> AEQVTKSVLFVCLGNICRSPIAEAVFRKLVTDQNISDNWVIDSGAVSDWNVGRSPDPRAVSCLRNHGINTAHKARQVTKEDFVTFDYILCMDESNLRDLNRKSN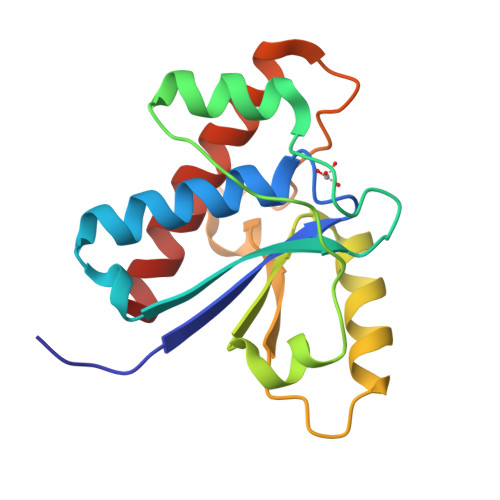QVKNCRAKIELLGSYDPQKQLIIEDPYYGNDADFETVYQQCVRCCRAFLEKVR>GSMAPRAGFDAEQVRDKARKDLLHLLEGVRGKKNLVIEKDLAGPLGVIVKASTLRDYGVDNFFFLENKNTGTSQRNIVFIARGESVRNAHAIAAQIKRIQRESQTSHDFHIFWVPRRTLFSDKVLEEAGVLGDANISELPLYFFPLERDVLSLELNDSFRDLYLAKDPTPVFLLSRALMGIQKKHGLFPRIIGKGENAKRVADLLSRMRQELLAGEEAGESDRAGLSPSTTIESVIIIDREVDFVTPLLTQLTYEGLIDEYFGIQNNQTDVDAVIVGAPAQSAASTSTAVPTNSSQSRKRKIQLDGSDSLYSQLRDANFAIVGSLLNTVARRLKSDYESRHNTKTTAELKEFVKKLPGYQAEQQSLKIHSNIAEEIINYTRTEIFNKLLEVQQNLAAGADPSSQFDSIEELVARDTPLPQVLRLLCLYSCISGGIKTKELDHFRRLVLQGYGHQHLLTLHNLERLQMFLSKSSPLASMITMSGSSGGPDQKTNYTYLRKQLRLIVDEVNEQDPNDIAYVYSGYAPLSIRLVQCVLQKQYLLSITKGSGTVIAAGPVAGGGAQGWKGFEEIVKHARGPTFDEIQKGEDKAVKARALLSGSSGDKKTVFVVFVGGITFTEIAALRFIAKQEEARRNIVICTTSIINGNRMMNAAIETATFEKTTVTTAAAQ[2x];>[2x]MGSSFEVIARTAYEEGRTRLATELLNHEPR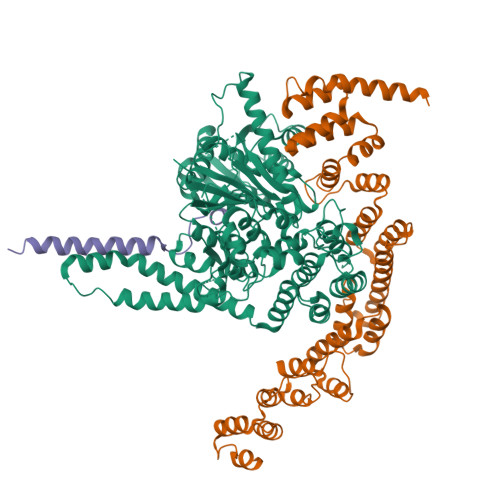AGRQVPLLLSMEEDELALDKAIESGDTDLIYFVIHQLRRKLPLASFFRVVSSRPTASAMVEALARNSDGDGNEDTALLKDLYYQDDRRLDGASVFIREALQQPETRTASDKLDLAANLLQGNQKEHVFELGALKEAKMLLRMQETFERDLTDSFVGLSVNQTMFKLIKLGYHGRAKKIQSEFKVPERVAWWIRLQALVAKRDWNEIEEISRQRKSPIGWEPFFNQVLQAGNPRLAATFIPKCTNLEPGQTITMYEKCGMRVKAAEEAVRLKDTEAWNRLLEAAGRNTAEGREIERLGATVFKK;>[2x]GSLILEREEEIRNIEQGVSDLNVLFQQVAQLVAEQGEVLDTIERNVEAVGDDTRGADRELRAAARYQ> MHHHHHHKNIVNTSILSIVYKKDDLIDLSRYGAKINIGDRVYYDSIDKNQIKLINLESSTIEVILKNAIVYNSMYENFSTSFWIKIPKYFSKINLNNEYTIINCIENNSGWKVSLNYGEIIWTLQDNKQNIQRVVFKYSQMVNISDYINRWIFVTITNNRLTKSKIYINGRLIDQKPISNLGNIHASNKIMFKLDGCRDPRRYIMIKYFNLFDKELNEKEIKDLYDSQSNSGILKDFWGNYLQYDKPYYMLNLFDPNKYVDV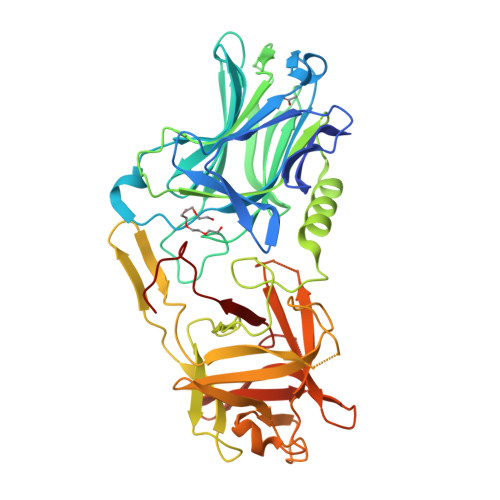NNIGIRGYMYLKGPRGSVVTTNIYLNSTLYEGTKFIIKKYASGNEDNIVRNNDRVYINVVVKNKEYRLATNASQAGVEKILSALEIPDVGNLSQVVVMKSKDDQGIRNKCKMNLQDNNGNDIGFIGFHLYDNIAKLVASNWYNRQVGKASRTFGCSWEFIPVDDGWGESSL>EPAAAPAPTKEEVLLTEIRDLLKEQNNRS[5x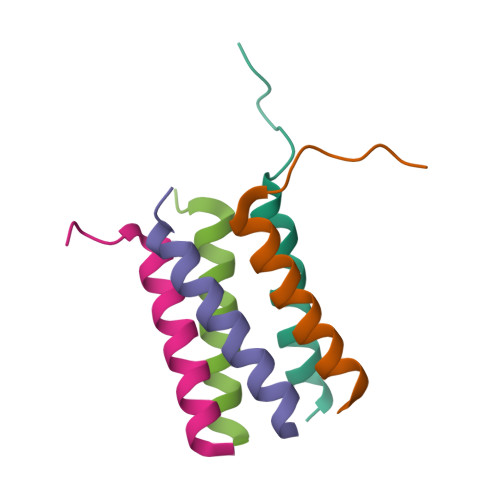]>SNAMMPDKKGYIIDID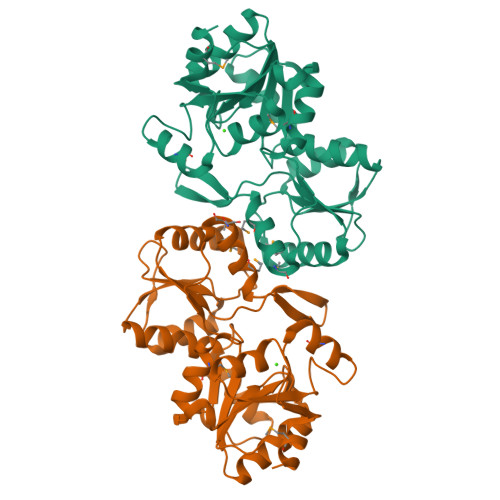GVIGKSVTPIPEGVEGVKKLKELGKKIIFVSNNSTRSRRILLERLRSFGLEVGEDEILVATYATARFIAREKPNAKVFTTGEEGLIEELRLAGLEIVDYDEAEYLVVGSNRKINFELMTKALRACLRGIRYIATNPDRIFPAEDGPIPGTGMIIGALYWMTGREPDVVVGKPSEVIMREALDILGLDAKDVAVVGDQIDVDVAAGKAIGAETVLVLTGVTTRENLDQMIERHGLKPDYVFNSLKDMVEALEG[4x]Alpha-hydroxy acids are oxidized by a family of FMN-dependent enzymes. These enzymes use molecular oxygen to convert their substrate to product with the liberation of H2O2 as a by-product. PaLCTO is annotated as lactate oxidase and its closest homolog in Pediococcus acidilactici proteome does not use lactate as a substrate. We describe here structural and biophysical studies of PaLCTO, which revealed FMN-dependent folding and oligomerization of the enzyme.

In order to study whether monomeric enzyme could incorporate the co-factor, we incubated it with FMN and subsequently carried out SEC analysis to see if the protein oligomerizes in the presence of the co-factor. The protein indeed eluted at the same elution volume as native tetrameric protein indicating co-factor dependent oligomerization. Refolded protein had similar spectra to WT native PaLCTO and melting temperature (47 ± 1°C). The structure was solved to 2.60 Å resolution. The structure proved that PaLCTO gains the same three-dimensional structure as WT PaLCTO when refolded. We also saw signs of two conformations for the chain S201 –A219 in the structure of refolded PaLCTO, but due to modest resolution and lack of electron density the chains could not be built. Like WT enzyme the refolded oligomer fitted well to the SAXS data. SAXS analysis of refolded PaLCTO were also in line and indicated that the protein had a molecular weight of 151 kDa, Kratky plot was similar to native PaLCTO and Dmax was 113 Å as for the native tetramer.

> SMTMINGYEQSDREEKIDILNLESLEKQAEEIIPAGGFGYIAGGSEDEWTLKQNRMAFHHRQIAPKALSGIEKPELNTEIFGIPLNTPVMMAPAAAQGLAHSQGEKDTARGLAAVGGLMAQSTYSSVSIAETAAAGGDAPQFFQLYMSKDWNFNESLLDEAKKANVKAIILTVDATVDGYREADIKNKFTFPLPMANLIKFSEGNGQGKGIEEIYASAAQNIRPEDVKRIADYTNLPVIVKGIQTPEDAIRAIDAGAAGIYVSNHGGRQLNGGPASFDVLEDIATAVNKQVPIIFDSGVRRGSDVFKALASGADLVALGRPVIYGLALGGAKGVQSVFEHLNHELEIVMQLAGTKTIEDVKNNSLLNIKY Periplasmic binding proteins (PBPs) are a class of proteins that participate in the cellular transport of various ligands. The structurally symmetric bilobal architecture of their fold has long been thought to originate from a duplication and fusion event of an individual lobe. Here, the crystal structures of two permuted halves of a modern ribose-binding protein (RBP) from Thermotoga maritima are reported.

RBP-CPN was designed to consist only of the βA–Eα1–4 elements, which are directly linked to α9. Similarly, RBP-CPC consists of the elements βF–Jα5–8 connected to α4 of RBP by permutation. An alternative explanation could be the formation of an interface between two crystallographic dimers, as indicated by an analysis with the PISA server. In this case, the C-terminal α8 would not originate from the same chain of the asymmetric unit but from its corresponding symmetry mate. The resulting extended arrangement is facilitated by an interaction of the βI strand and the residue stretch 116′–120′. The central β-sheet as well as all α-helices appear to be well ordered, except for the loops close to the unresolved region and the termini. The r.m.s.d. of 0.5 Å over 135 Cα atoms of the resolved residues, however, indicates a high similarity between RBP-CPC and the corresponding elements of full-length RBP. However, it appears that RBP-CPC, which still contains this corresponding helix 8, does not reliably form a dimer.

>[2x]MKEIPYAELLGILSAQPTWDRSNGFHSVVDQYPEFKMVAQQSAEFDRDTAYKVTEQILQAHPEIKAIWCGNDAMALGAMKACEAAGRTDIYIFGFDGAEDVINAIKEGKQIVATIMVGHNHNYYGGVLAGEYFVKFLKEKYPDGGHHHHHH> MAIGLKAYPELC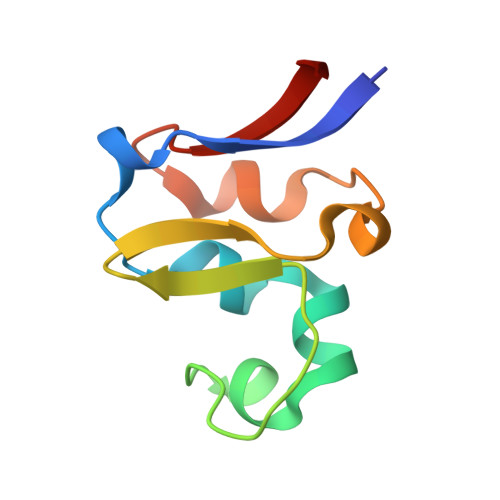HGCGNCVIACPVNALRSPEVAGGKGPTDDVEIIMIVEDGVVNIKNPDLCGKCGTCVESCPVDAIRLEELE>WRGSHHHHHHGSACASGKKDTTSGQKLKVVATNSIIADITKNIAGDKIDLHSIVPIGQDPHEYEPLPEDVKKTSEADLIFYNGINLETGGNAW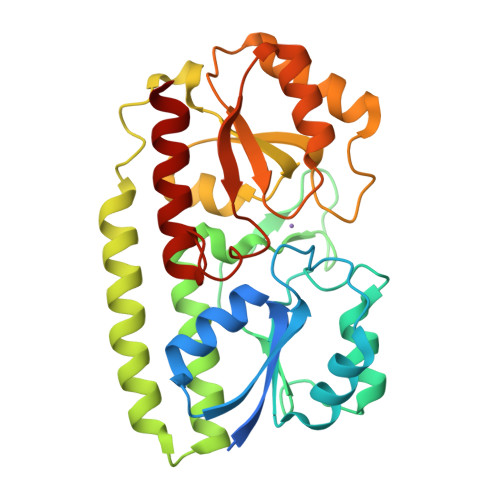FTKLVENAKKTENKDYFAVSDGVDVIYLEGQNEKGKEDPHAWLNLENGIIFAKNIAKQLSAKDPNNKEFYEKNLKEYTDKLDKLDKESKDKFNKIPAEKKLIVTSEGAFKYFSKAYGVPSAYIWEINTEEEGTPEQIKTLVEKLRQTKVPSLFVESSVDDRPMKTVSQDTNIPIYAQIFTDSIAEQGKEGDSYYSMMKYNLDKIAEGLAK[4x]Ras suppressor protein 1 (Rsu1), a leucine-rich repeat (LRR)-containing protein conserved from human to worms, was recognized as a major FA component and is important for FA formation and cell motility. Among the IAC components, tripartite integrin-linked kinase (ILK) associates with another two key players PINCH and Parvin to form the ILK/PINCH/Parvin (IPP) complex, which acts as an essential platform to recruit many proteins for the FA formation and signaling and provide a linkage between FA and actin cytoskeleton. Here, we solved the crystal structures of the Rsu1/PINCH1 complex and found that Rsu1 strongly binds to PINCH1 through a large concave surface on its LRR solenoid. The cellular data supported the inhibitory effect of Rsu1 on the IPP complex. These results indicated that Rsu1, by interacting with PINCH1 and preventing PINCH1 from binding to actin, modulates actin dynamics at the FA and thereby regulates the stress fiber formation and cell adhesion dynamics.

We prepared the Rsu1/PINCH1 complex by combinatorial usage of the purified fragments that contains the elements necessary and sufficient for the Rsu1/PINCH1 interaction and successfully obtained the crystals of the Rsu1ΔC/PINCH1_LIM5C and Rsu1/PINCH1_LIM45C complexes. The complex structures of Rsu1ΔC/PINCH1_LIM5C with one crystal form at 1.65 Å resolution and Rsu1/PINCH1_LIM45C with two different crystal forms at 2.2 Å and 3.15 Å resolution respectively were determined by the molecular replacement method. In the Rsu1/PINCH1_LIM45C complex, the nine LRRs of Rsu1 form a curved solenoid capped by the helical regions in the both N- and C-termini, named N-cap and C-cap, respectively. The N-cap consists of the α1-helix while the C-cap contains three α-helices (α2–4). Both the two helical regions cap the LRR-solenoid by forming extensive hydrophobic interactions with LRR1–2 and LRR8–9, respectively. Although lacking the C-terminal half of the LRR-motif, LRR9 remains folded presumably due to the presence of the C-cap. Consistent with our biochemical finding, the LRR-solenoid of Rsu1 interacts with both the LIM5 domain and the C-terminal tail (C-tail, folded as a α-helix) of PINCH1 through the concave surface of the solenoid, mainly formed by the parallel β-sheet and the flanking loop regions. In all three complex structures that we solved, the LIM5C fragment in PINCH1 and the LRRs in Rsu1 showed the essentially same conformation with the overall RMSD of ~0.3 Å. However, the LIM4 domain in PINCH1 adopts different orientations as observed in the two crystal forms of the Rsu1/PINCH1_LIM45C complex, indicating the intrinsic, structural flexibility between the LIM4 and LIM5 domains. The full-length structure of Rsu1 that we solved also provides a valuable information to uncover other binding partner(s) of Rsu1.

> GAMGSMSKSLKKLVEESREKNQPEVDMSDRGISNMLDVNGLFTLSHITQLVLSHNKLTMVPPNIAELKNLEVLNFFNNQIEELPTQISSLQKLKHLNLGMNRLNTLPRGFGSLPALEVLDLTYNNLSENSLPGNFFYLTTLRALYLSDNDFEILPPDIGKLTKLQILSLRDNDLISLPKEIGELTQLKELHIQGNRLTVLPPELGNLDLTGQKQVFKAENNPWVTPIADQFQLGVSHVFEYIRSETYKYLYGRHMQANPEPPKKNNDKSKKISRKPLAAKNR;> GPGSMGVPICGACRRPIEGRVVNAMGKQWHVEHFVCAKCEKPFLGHRHYERKGLAYCETHYNQLFGDVCFHCNRVIEGDVVSALNKAWCVNCFACSTCNTKLTLKNKFVEFDMKPVCKKCYEKFPLELKKRLKKLAETLGRK> MEGERKNNNKRWYFTREQLENSPSRRFGVDPDKELSYRQQAANLLQDMGQRLNVSQLTINTAIVYMHRFYMIQSFTRFPGNSVAPAALFLAAKVEGQPKKLEHVIKVAHTCLHPQESLPDTRSEAYLQQVQDLVILESIILQTLGFELTIDHPHTHVVKCTQLVRASKDLAQTSYFMATNSLHLTTFSLQYTPPVVACVCIHLACKWSNWEIPVSTDGKHWWEYVDATVTLELLDELTHELLQILEKTPNRLKRIWNWRACEAAKKTKADDRGTDEKTSEQTILNMISQSSSDTTIAGLMSMSTSTTSAVPSLPVSEESSSNLTSVEMLPGKRWLSSQPSFKLEPTQGHRTSENLALTGVDHSLPQDGSNAFISQKQNSKSVPSAKVSLKEYRAKHAEELAAQKRQLENMEANVKSQYAYAAQNLLSHHDSHSSVILKMPIEGSENPERPFLEKADKTALKMRIPVAGGDKAASSKPEEIKMRIKVHAAADKHNSVEDSVTKSREHKEKHKTHPSNHHHHHNHHSHKHS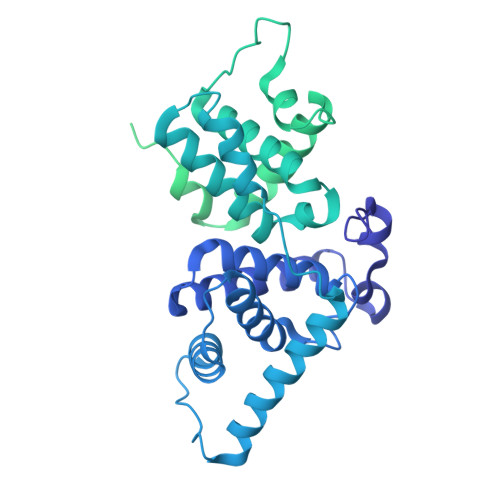HSQLPVGTGNKRPGDPKHSSQTSNLAHKTYSLSSSFSSSSSTRKRGPSEETGGAVFDHPAKIAKSTKSSSLNFSFPSLPTMGQMPGHSSDTSGLSFSQPSCKTRVPHSKLDKGPTGANGHNTTQTIDYQDTVNMLHSLLSAQGVQPTQPTAFEFVRPYSDYLNPRSGGISSRSGNTDKPRPPPLPSEPPPPLPPLPK>GSFTSTSLSDQKYLSSSSSSSSNADPNKRIFQAYGNAAALFVQMGAYRGGPTTFAVVGLASKPIHVFRLPWYKCEWISNNGSSIRAKAYKMLPDWGYGRVYTVVVVNCTFPVNPNQDNAGGRLMLNAYYDESQRKYEKFTALEELPGSYNESKFRPPYQYEYLYCGSSLYGNLSASRFREWMAYHAWFFGPSSHFVFHDAGGVSPEVRAALDPWVRAGRATVQDIRGQAEFDGYYYNQFLVVNDCLHRYRYSANWTFYFDVDEYIYLPEGNTLESVLKDFSNYTQFTIEQNPMSSALCFNDSTQDYPRQWGFEKLLFRESRTGIRRDRKYAIQAKNAYATGVHMSENVIGKTLHQTETKIRYYHYHNSIQVPGELCREFLPLSAKNNVTWYNGLPYVYDDNMKKLASTIKDFERNT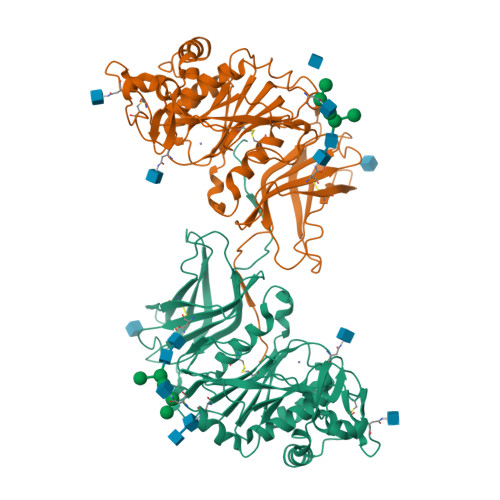IGNVQAYS[2x]> PIEVNDDCMACEACVEICPDVFEMNEEGDKAVVINPDSDLDCV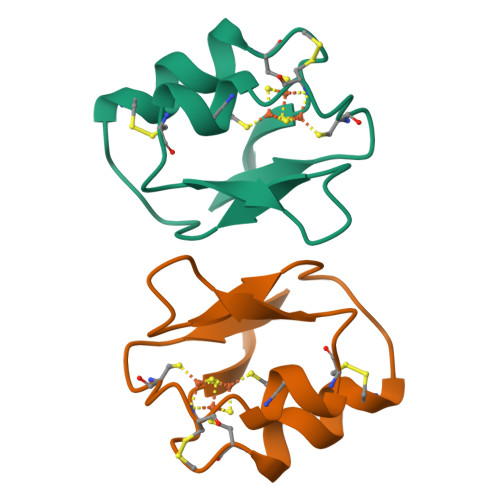EEAIDSCPAEAIVRS> MNVIAILNHMGVYFKEEPIRELHRALERLNFQIVYPNDRDDLLKLIENNARLCGVIFDWDKYNLELCEEISKMNENLPLYAFANTYSTLDVSLNDLRLQISFFEYALGAAEDIANKIKQTTDEYINTILPPLTKALFKYVREGKYTFCTPGHMGGTAFQKSPVGSLFYDFFGPNTMKSDISISVSELGSLLDHSGPHKEAEQYIARVFNADRSYMVTNGTSTANKIVGMYSAPAGSTILIDRNCHKSLTHLMMMSDVTPIYFRPTRNAYGILGGIPQSEFQHATIAKRVKETPNATWPVHAVITNSTYDGLLYNTDFIKKTLDVKSIHFDSAWVPYTNFSPIYEGKCGMSGGRVEGKVIYETQSTHKLLAAFSQASMIHVKGDVNEETFNEAYMMHTTTSPHYGIVASTETAAAMMKGNAGKRLINGSIERAIKFRKEIKRLRTESDGWFFDVWQPDHIDTTECWPLRSDSTWHGFKNIDNEHMYLDPIKV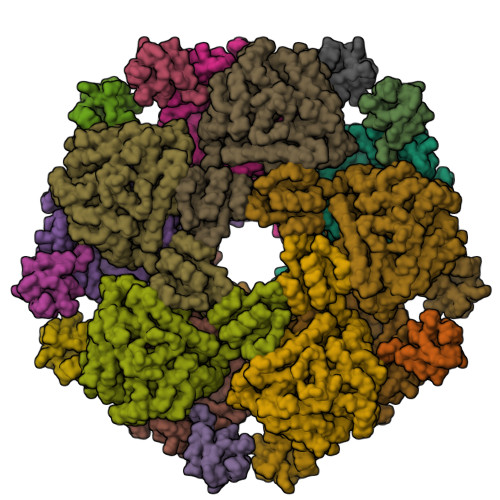TLLTPGMEKDGTMSDFGIPASIVAKYLDEHGIVVEKTGPYNLLFLFSIGIDKTKALSLLRALTDFKRAFDLNLRVKNMLPSLYREDPEFYENMRIQELAQNIHKLIVHHNLPDLMYRAFEVLPTMVMTPYAAFQKELHGMTEEVYLDEMVGRINANMILPYPPGVPLVMPGEMITEESRPVLEFLQMLCEIGAHYPGFETDIHGAYRQADGRYTVKVLKE;> DKTALTVIRLGGIFSRRQQYQLPVNVTASTLTLLLQKPLKLHDMEVVHISFERSALEQWLSKGGEIRGKLNGIGFAQKLNLEVDSAQHLVVRDVSLQGSTLALPGS> KPEPTDEEWELIKTVTEAHVATNAQGSHWKQKRKFLPEDIGQAPIVNAPEGGKDDLEAFSHFTKIITPAITRVVDFAKKLPMFCELPCEDQIILLKGCCMEIMSLRAAVRYDPESETLTLNGEMAVTRGQLKNGGLGVVSDAIFDLGMSLSSFNLDDTEVALLQAVLLMSSD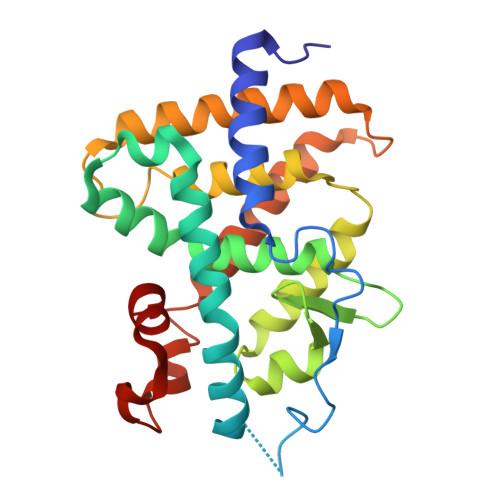RPGLACVERIEKYQDSFLLAFEHYINYRKHHVTHFWPKLLMKVTDLRMIGACHASRFLHMKVECPTELFPPLFLEVFE> MPSFDEALQRVGEFGRFQRRVFLLLCLTGVTFAFLFVGVVFLGTQPDHYW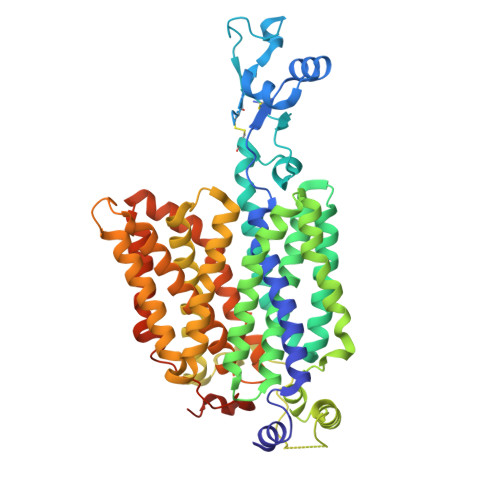CRGPSAAALAERCGWSPEEEWNRTAPASRGPEPPERRGRCQRYLLEAANDSASATSALSCADPLAAFPNRSAPLVPCRGGWRYAQAHSTIVSEFDLVCVNAWMLDLTQAILNLGFLTGAFTLGYAADRYGRIVIYLLSCLGVGVTGVVVAFAPNFPVFVIFRFLQGVFGKGTWMTCYVIVTEIVGSKQRRIVGIVIQMFFTLGIIILPGIAYFIPNWQGIQLAITLPSFLFLLYYWVVPESPRWLITRKKGDKALQILRRIAKCNGKYLSSNYSEITVTDEEVSNPSFLDLVRTPQMRKCTLILMFAWFTSAVVYQGLVMRLGIIGGNLYIDFFISGVVELPGALLILLTIERLGRRLPFAASNIVAGVACLVTAFLPEGIAWLRTTVATLGRLGITMAFEIVYLVNSELYPTTLRNFGVSLCSGLCDFGGIIAPFLLFRLAAVWLELPLIIFGILASICGGLVMLLPETKGIALPETVDDVEKLGSPHSCKCGRNKKTPVSRSHL1-methyl-4-[(1E)-3-(3-methyl-1,3-benzothiazol-3-ium-2-yl)prop-1-en-1-yl]quinolin-1-ium 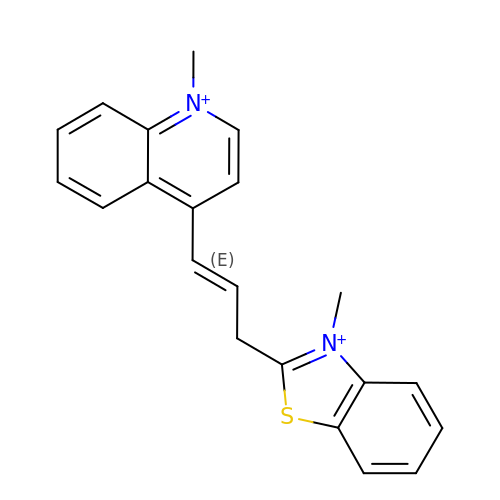| C21 H20 N2 S | BUHZEFGMJCIGHQ-BQYQJAHWSA-N6-{[(3R,4R)-4-(2-{[(2S)-1-(3-fluorophenyl)propan-2-yl]amino}ethoxy)pyrrolidin-3-yl]methyl}-4-methylpyridin-2-amine 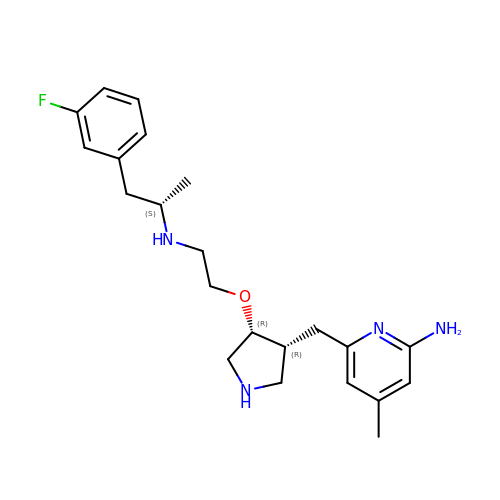| C22 H31 F N4 O | AUSIEXNWJKDTQY-CDXJDZJCSA-N> PLGSRKCEKAGCTATCPVCFASASERCAKNGYTSRWYHLSCGEHFCNECFDHYYRSHKDGYDKYTTWKKIWTSNGKTEPSPKAFMADQQLPYWV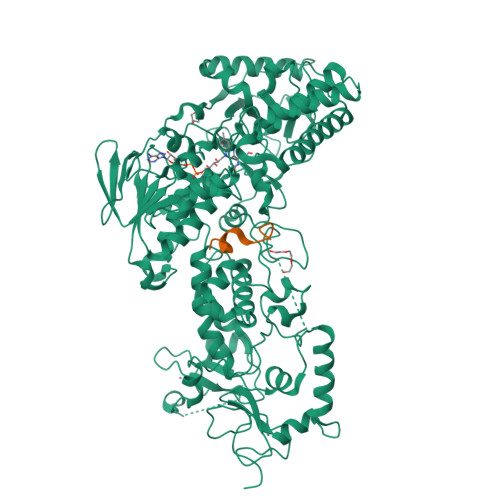QCTKPECRKWRQLTKEIQLTPQIAKTYRCGMKPNTAIKPETSDHCSLPEDLRVLEVSNHWWYSMLILPPLLKDSVAAPLLSAYYPDCVGMSPSCTSTNRAAATGNASPGKLEHSKAALSVHVPGMNRYFQPFYQPNECGKALCVRPDVMELDELYEFPEYSRDPTMYLALRNLILALWYTNCKEALTPQKCIPHIIVRGLVRIRCVQEVERILYFMTRKGLINTGVLSVGADQYLLPKDYHNKSVIIIGAGPAGLAAARQLHNFGIKVTVLEAKDRIGGRVWDDKSFKGVTVGRGAQIVNGCINNPVALMCEQLGISMHKFGERCDLIQEGGRITDPTIDKRMDFHFNALLDVVSEWRKDKTQLQDVPLGEKIEEIYKAFIKESGIQFSELEGQVLQFHLSNLEYACGSNLHQVSARSWDHNEFFAQFAGDHTLLTPGYSVIIEKLAEGLDIQLKSPVQCIDYSGDEVQVTTTDGTGYSAQKVLVTVPLALLQKGAIQFNPPLSEKKMKAINSLGAGIIEKIALQFPYRFWDSKVQGADFFGHVPPSASKRGLFAVFYDMDPQKKHSVLMSVIAGEAVASVRTLDDKQVLQQCMATLRELFKEQEVPDPTKYFVTRWSTDPWIQMAYSFVKTGGSGEAYDIIAEDIQGTVFFAGEATNRHFPQTVTGAYLSGVREASKIAAF;> PLGSPEFSERGSKSPLKRAQEQSPRKRGRPPKDEKDLTIPESSTVKGMMAGPMAAFKWQPTASEPVKDADPHFHHFLLSQTEKPAVCYQAITKKLKICEEETGSTSIQAADSTAVNGSITPTDK>[2x]MLPQRLHPSRLLALALFSLVLGLAGCQTKPPQTGLSAEQIAVLQEQGSELRDEGWEFGMSSKVLFGNNLDRLNPDSRNTLT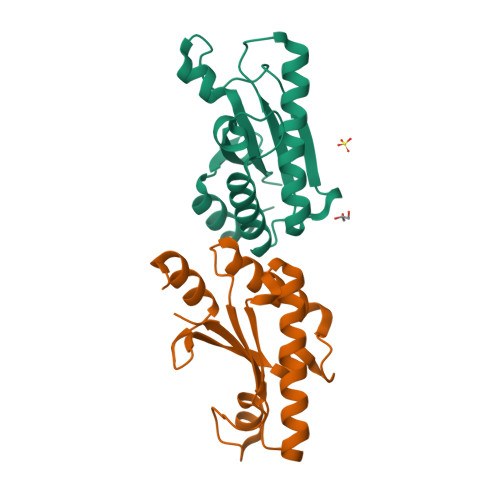KIARALLAVDIDKVRLEGHTDNYGDEGYNQKLSERRAESVAAVFREAGMPAANIEVRGLGMSKPVADNKTRAGRSENRRVAIIVPAE>GHMHTPFIVALDFPSKQEVERFLRPFAGTPLFVKVGMELYYQEGPAIVAFLKEQGHAVFLDLKLHDIPNTVKQAMKGLARVGADLVNVHAAGGRRMMEAAIEGLDAGTPSGRMRPRCIAVTQLTSTDERMLHEELWISRPLVETVAHYAALAKESGLDGVVCSANEAAFIKERCGASFLAVTP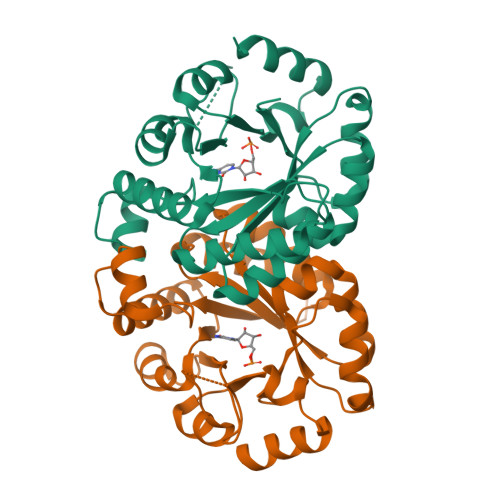GIRFADDAAHDQVRVVTPRKARALGSDYIVIGRSLTRAADPLRTYARLQHEWNGGERESTTPT[2x]The protein SidK, secreted by Legionella pneumophila, interacts with the V-ATPase to inhibit acidification of the phagolysosome in the early stages of infection. V-ATPases pump protons across a phospholipid membrane using energy from the hydrolysis of adenosine triphosphate (ATP) to adenosine diphosphate (ADP) and inorganic phosphate. Successful pathogens can subvert host defenses by secreting effectors that target V-ATPases to inhibit lysosomal acidification or lysosomal fusion with other cell compartments. This study reveals the structure of the V-ATPase:SidK complex, an assembly formed from the interaction of host and pathogen proteins involved in the infection of phagocytic white blood cells by Legionella pneumophila. Removal of the C-terminal residues 415–573 of SidK did not significantly affect V-ATPase inhibition by the SidK mutants, but truncations of the N-terminal region of the protein has been demonstrated to prevent V-ATPase inhibition. These data show that binding of the N-terminal domain of SidK to the V-ATPase is responsible for its partial yet specific inhibition of V-ATPase activity.

One SidK construct, consisting of residues 16–278 (SidK-N), yielded two crystal forms that diffracted X-rays to 2.3 to 2.4 Å resolution and the structure of SidK-N was determined from these crystals. The first crystal form contained one molecule of SidK(16–278) in the asymmetric unit and the final model included amino acids 16–274. The protein has an elongated and slightly bent α-helical structure consisting of three α-helical bundles. The three α-helical bundles contain four, four, and three α-helices, respectively, and are connected by loops in the bundles. The first α-helical bundle (α1–2, α5–6) also has an extension nearly perpendicular to the bundle axis that consists of two additional short α-helices (α3-α4) (green arrowheads). However, the N-terminal bundle with its extensions, which from previous analysis was proposed to be the region that interacts with the V-ATPase, does not resemble any other known protein structures. The monomeric SidK predominates in solution, even at high concentrations, and therefore the elongated monomer structure is expected to be the functional state of the protein. Only the N-terminal region of SidK interacts with the V-ATPase and consequently a highly-elongated SidK structure was unexpected. Mapping the contact surfaces in all three SidK:A-subunit pairs in the cryo-EM map to the SidK crystal structure, the main contact surface appears to involve residues Gly24, Tyr28, Phe62, Ser85, and Trp122 from the first α-helical bundle of SidK.

> SNAEQYHSQVVGKIGYIARCMQTIDPENNLKKIREDYQDVLIWAEKNYRFEEILEASKSGKCPNDLDALSRRSLILQELLRLVSSISPFKMKLDLIESQYEKMKQHVNLWKSDYHVKLNQLNQLTDYLKNAAPTPKNNFLRAMTSVLQMQIAQYGITEDNEGINQLFKLGLHLLAMANEKIDEQYHLFKGYVKDQPEESPFEGILPAEDQKILVKTMIDYAMPKLSSKVLQDKLSALSSSDVLTKTLLDSIDRIVKENEKLNALSK> MSFVGKKYKLDKSENFDEYMKELGVGLVTRKMGNSLSPTVEVTLEGDTYTLTTTSTFKTSAISFKLGVEFDEETLDGRNVKSIITLDGNKLTQEQKGDKPTTIVREFTDNELITTLTIGNVKCVR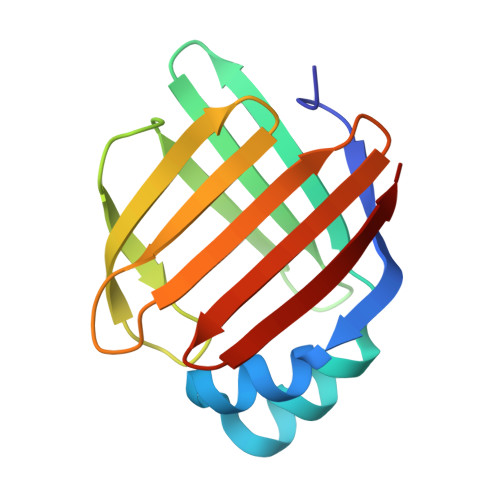VYKAV6-(2-{6-[2-(2-amino-6-methylpyridin-4-yl)ethyl]pyridin-2-yl}ethyl)-4-methylpyridin-2-amine | C21 H25 N5 | 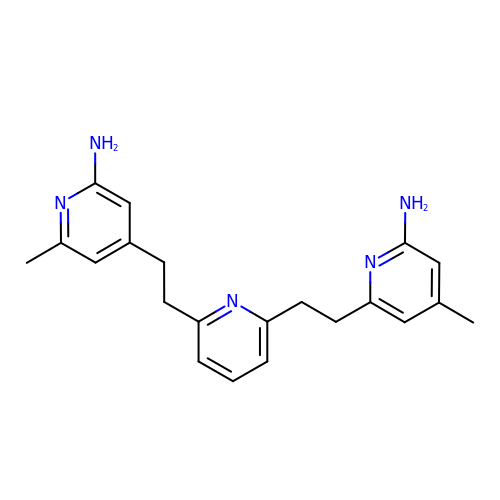ZMKGFXFDYMNDSP-UHFFFAOYSA-N>DYKDDDDKLVPRGSCHPRLSLHRPALEDLLLGSEANLTCTLTGLRDASGATFTWTPSSGKSAVQGPPERDLCGCYSVSSVLPGCAQPWNHGETFTCTAAHPELKTPLTANITKSGNTFRPEVHLLPPPSEELALNELVTLTCLARGFSPKDVLVRWLQGSQELPREKYLTWASRQEPSQGTTTYAVTSILRVAAEDWKKGETFSCMVGHEALPLAFTQKTIDRLAGKPTHINVSVVMAEADGTCY[10x];> KSPIFGPEEVNSVEGNSVSITCYYPPTSVNRHTRKYWCRQGARGGCITLISSEGYVSSKYAGRANLTNFPENGTFVVNIAQLSQDDSGRYKCGLGINSRGLSFDVSLEVSQGPGLLNDTKVYTVDLGRTVTINCPFKTENAQKRKSLYKQIGLYPVLVIDSSGYVNPNYTGRIRLDIQGTGQLLFSVVINQLRLSDAGQYLCQAGDDSNSNKKNADLQVLKPEPELVYEDLRGSVTFHCALGPEVANVAKFLCRQSSGENCDVVVNTLGKRAPAFEGRILLNPQDKDGSFSVVITGLRKEDAGRYLCGAHSDGQLQEGSPIQAWQLFVNEESTIPRSPTVVKGVAGGSVAVLCPYNRKESKSIKYWCLWEGAQNGRCPLLVDSEGWVKAQYEGRLSLLEEPGNGTFTVILNQLTSRDAGFYWCLTNGDTLWRTTVEIKIIEGEPNLKVPGNVTAVLGETLKVPCHFPCKFSSYEKYWCKWNNTGCQALPSQDEGPSKAFVNCDENSRLVSLTLNLVTRADEGWYWCGVKQGHFYGETAAVYVAVEERKAAGSRDVSLAKAD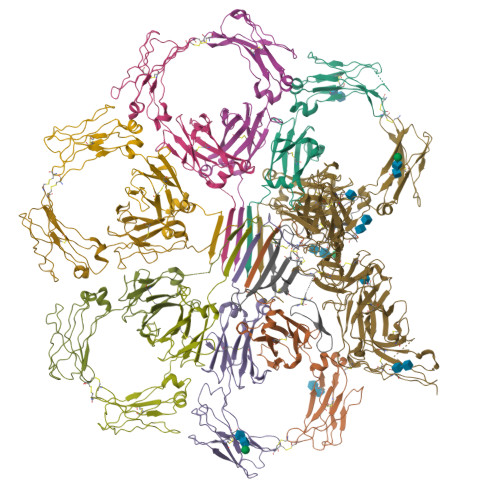AAPDEKVLDSGFREIENKAIQDPRHHHHHH;> QEDERIVLVDNKCKCARITSRIIRSSEDPNEDIVERNIRIIVPLNNRENISDPTSPLRTRFVYHLSDLCKKCDPTEVELDNQIVTATQSNICDEDSATETCYTYDRNKCYTAVVPLVYGGETKMVETALTPDACYPD> MVKLTAELIEQAAQYTNAV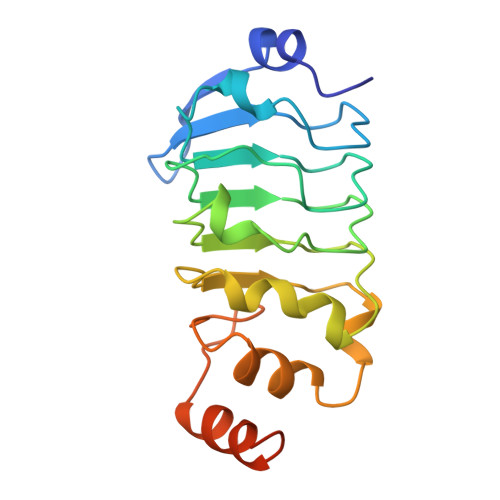RDRELDLRGYKIPVIENLGATLDQFDAIDFSDNEIRKLDGFPLLRRLKTLLVNNNRICRIGEGLDQALPDLTELILTNNSLVELGDLDPLASLKSLTYLCILRNPVTNKKHYRLYVIYKVPQVRVLDFQKVKLKERQEAEKMFKGKRGAQLAKDIAR>DWPVYHRIDGPIVMIGFGSIGRGTLPLIERHFAFDRSKLVVIDPSDEARKLAEARGVRFIQQAVTRDNYRELLVPLLTAGPGQGFCVNLSVDTSSLDIMELARENGALYIDTVVEPWLGFYFDPDLKPEARSNYALRETVLAARRNKPGGTTAVSCCGANPGMVSWFVKQALVNLAADLGVTGEEPTTREEWARLAMDLGVKGIHIAERDTQRASFPKPFDVFVNTWSVEGFVSEGLQPAELGWGTFERWMPDNARGHDSGCGAGIYLLQPGANTRVRSWTPTAMAQYGFLVTHNESISIADFLTVRDAAGQAVYRPTCHYAYHPCNDAVLSLHEMFGSGKRQSDWRILDETEIVDGIDELGVLLYGHGKNAYWYGSQLSIEETRRIAPDQNATGLQVSSAVLAGMVWALENPNAGIVEADDLDFRRCLEVQTPYLGPVVGVYTDWTPLAGRPGLF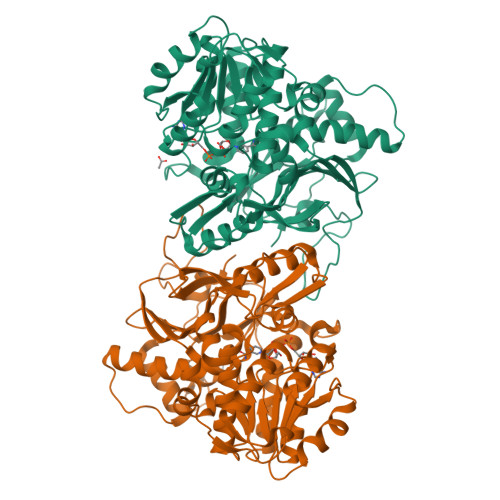PEDIDTSDPWQFRNVLVR[2x]>[4x]GHMEETFSKPNLSAKDLALLLFTHLPGNNTPFHILAQVLSKIAYKSGKSGAFLDAF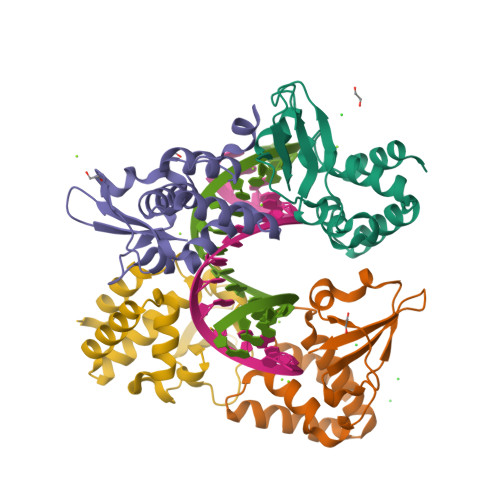HQILSEGENAQAALTRLSRTFDAFMGVVPPVIRVKNFQTVPRPCQKSLRAVPPNPTIDKGWVCVYSSEQGETRALKI>CCC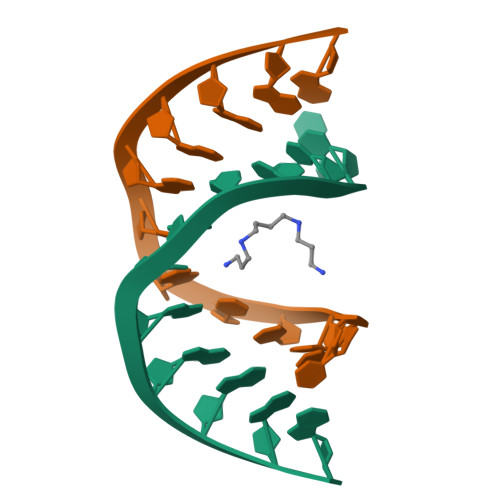CCGCGGGGG[2x]>MSFEGARLSMRSRRNGTMGSTRTLYSSVSRSTDVSYSDSDLVNFIQANFKKRECVFFTRDSKAMENICKCGYAQSQHIEGTQINQNEKWNYKKHTKEFPTDAFGDIQFETLGKKGKYLRLSCDTDSETLYELLTQHWHLKTPNLVISVTGGAKNFALKPRMRKIFSRLIYIAQSKGAWILTGGTHYGLMKYIGEVVRDNTISRNSEENIVAIGIAAWGMVSNRDTLIRSCDDEGHFSAQYIMDDFTRDPLYILDNNHTHLLLVDNGCHGHPTVEAKLRNQLEKYISERTSQDSNYGGKIPIVCFAQGGGRETLKAINTSVKSKIPCVVVEGSGQIADVIASLVEVEDVLTSSMVKEKLVRFLPRTVSRLPEEEIESWIKWLKEILESSHLLTVIKMEEAGDEIVSNAISYALYKAFSTNEQDKDNWNGQLKLLLEWNQLDLASDEIFTNDRRWESADLQEVMFTALIKDRPKFVRLFLENGLNLQKFLTNE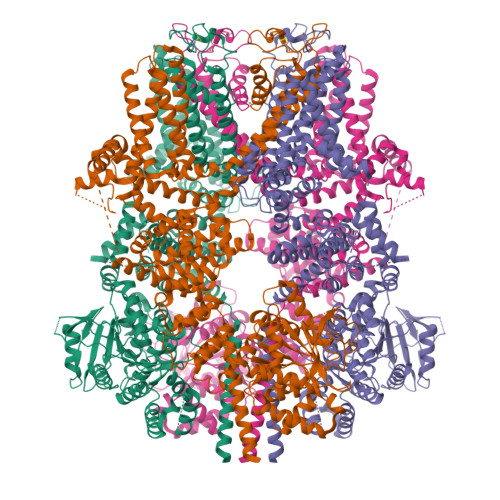VLTELFSTHFSTLVYRNLQIAKNSYNDALLTFVWKLVANFRRSFWKEDRSSREDLDVELHDASLTTRHPLQALFIWAILQNKKELSKVIWEQTKGCTLAALGASKLLKTLAKVKNDINAAGESEELANEYETRAVELFTECYSNDEDLAEQLLVYSCEAWGGSNCLELAVEATDQHFIAQPGVQNFLSKQWYGEISRDTKNWKIILCLFIIPLVGCGLVSFRKKPIDKHKKLLWYYVAFFTSPFVVFSWNVVFYIAFLLLFAYVLLMDFHSVPHTPELILYALVFVLFCDEVRQWYMNGVNYFTDLWNVMDTLGLFYFIAGIVFRLHSSNKSSLYSGRVIFCLDYIIFTLRLIHIFTVSRNLGPKIIMLQRMLIDVFFFLFLFAVWMVAFGVARQGILRQNEQRWRWIFRSVIYEPYLAMFGQVPSDVDSTTYDFSHCTFSGNESKPLCVELDEHNLPRFPEWITIPLVCIYMLSTNILLVNLLVAMFGYTVGIVQENNDQVWKFQRYFLVQEYCNRLNIPFPFVVFAYFYMVVKKCFKCCCKEKNMESNACCFRNEDNETLAWEGVMKENYLVKINTKANDNSEEMRHRFRQLDSKLNDLKSLLKEIANNIKLEGGSSGGWSHPQFEK[4x]>[3x]MSPTAKPNSQVSLNQESV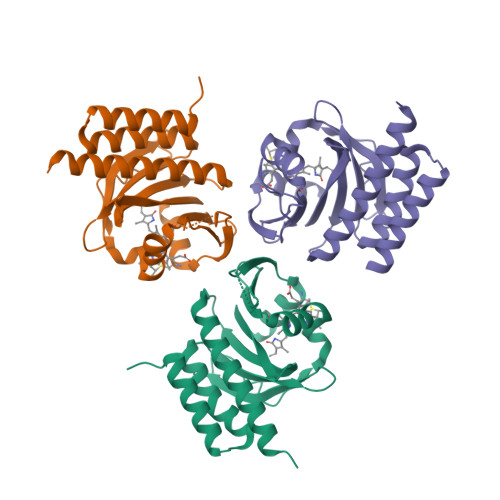LRRITARIRQSLELEDIITATTAEVRALLGTDRVMIYKFHPDGSGQVIAESIHENRLPSLLGLNFPADDIPPQARELLVKSKVRSIVDVATGMIGQSPVHDLETGELISEDICYRPVDSCHVEYLTAMGVKSSVVAPIFCQDELWGLLVSHHSENRTVSEDELEAMQMIVDQLAVAIAQSHLEHHHHHH> GPQSEPELKLESVVIVSRHGVRAPTKATQLMQDVTP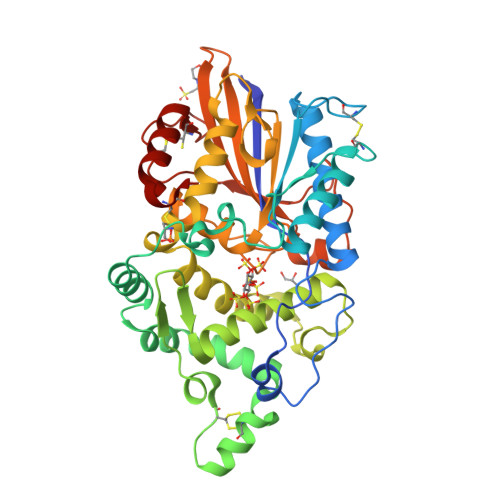DAWPTWPVKLGWLTPRGGELIAYLGHYQRQRLVADGLLAKKGCPQSGQVAIIADVDERTRKTGEAFAAGLAPDCAITVHTQADTSSPDPLFNPLKTGVCQLDNANVTDAILSRAGGSIADFTGHRQTAFRELERVLNFPQSNLCLKREKQDESCSLTQALPSELKVSADNVSLTGAVSLASMLTEIFLLQQAQGMPEPGWGRITDSHQWNTLLSLHNAQFYLLQRTPEVARSRATPLLDLIKTALTPHPPQKQAYGVTLPTSVLFIAGHAENLANLGGALELNWTLPGQPDNTPPGGELVFERWRRLSDNSQWIQVSLVFQTLQQMRDKTPLSLNTPPGEVKLTLAGCEERNAQGMCSLAGFTQIVNEARIPACSL> VIK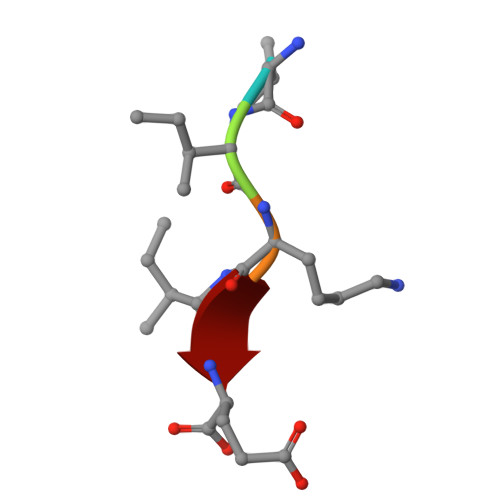IE> MPFTLGQRWISDTESELGLGTVVAVDARTVTLLFPSTGENRLYARSDSPVTRVMFNPGDTITSHDGWQMQVEEVKEENGLLTYIGTRLDTEESGVALREVFLDSKLVFSKPQDRLFAGQIDRMDRFALRYRARKYSSEQFRMPYSGLRGQRTSLIPHQLNIAHDVGRRHAPRVLLADEVGLGKTIEAGMILHQQLLSGAAERVLIIVPETLQHQWLVEMLRRFNLRFALFDDERYAEAQHDAYNPFDTEQLVICSLDFARRSKQRLEHLCEAEWDLLVVDEAHHLVWSEDAPSREYQAIEQLAEHVPGVLLLTATPEQLGMESHFARLRLLDPNRFHDFAQFVEEQKNYRPVADAVAMLLAGNKLSNDELNMLGEMIGEQDIEPLLQAANSDSEDAQSARQELVSMLMDRHGTSRVLFRNTRNGVKGFPKRELHTIKLPLPTQYQTAIKVSGIMGARKSAEDRARDMLYPE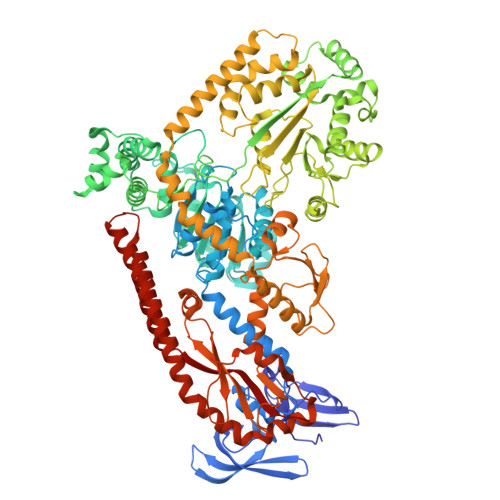RIYQEFEGDNATWWNFDPRVEWLMGYLTSHRSQKVLVICAKAATALQLEQVLREREGIRAAVFHEGMSIIERDRAAAWFAEEDTGAQVLLCSEIGSEGRNFQFASHMVMFDLPFNPDLLEQRIGRLDRIGQAHDIQIHVPYLEKTAQSVLVRWYHEGLDAFEHTCPTGRTIYDSVYNDLINYLASPDQTEGFDDLIKNCREQHEALKAQLEQGRDRLLEIHSNGGEKAQALAESIEEQDDDTNLIAFAMNLFDIIGINQDDRGDNMIVLTPSDHMLVPDFPGLSEDGITITFDREVALAREDAQFITWEHPLIRNGLDLILSGDTGSSTISLLKNKALPVGTLLVELIYVVEAQAPKQLQLNRFLPPTPVRMLLDKNGNNLAAQVEFETFNRQLNAVNRHTGSKLVNAVQQDVHAILQLGEAQIEKSARALIDAARNEADEKLSAELSRLEALRAVNPNIRDDELTAIESNRQQVMESLDQAGWRLDALRLIVVTHQ>RRA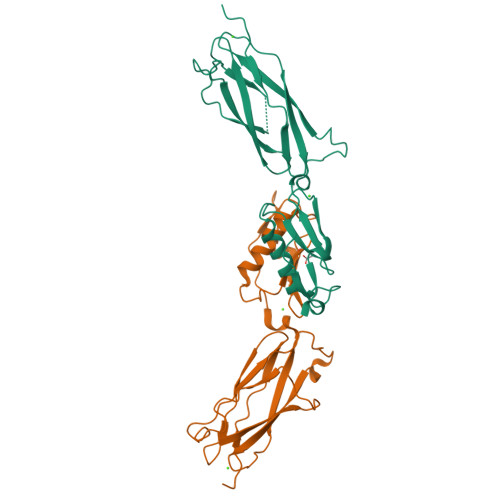TDTTPPTITVPSDIIAYRGEEFEFYFEITDDSGQVKNIELSTFGKPLGLNWLEYSEDNFNVPGNATSDNPLRVRVHGTVPLNEPIPADKNRAQFTETIRAWDAAGNVSSNITFVIKYRAQTDKYNPADPTITYVDRLSSLSPSEKNAVEAAVRAANPQIPAAARITVSANGTVTITYPDSSTDTITANRVVKDLASSR[4x]> NTYQFKNMIQCTVPKRSWWDFA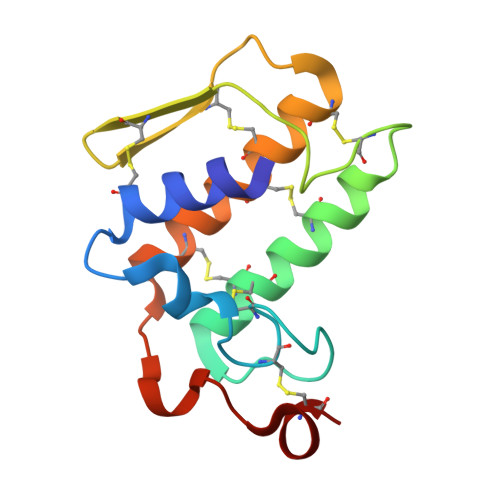DYGCYCGRGGSGTPIDDLDRCCQVHDNCYNSAREQGGCRPKQKTYSYECKAGTLSCSGSNNSCAATVCDCDRLAAICFAGAPYNDNNYNIDLKARCQ> MTDEEKVKAMRLARAIASDISLYNEQKIIKGIEQDNLFEVLKEELEEGRELYKSRVSQEIFTKMNFFERAINDIVLRSK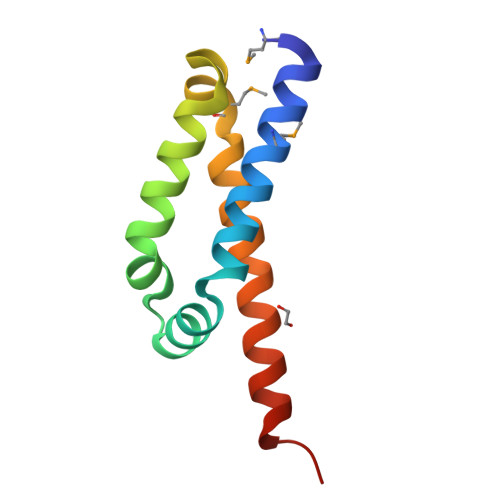AHVKSKIWGSHHHHHH> VVMSRGRIPRLGAAVLVALTTAAAACGADSQGLVVSFYTPATDGATFTAIAQRCNQQFGGRFTIAQVSLPRSPNEQRLQLARRLTGNDRTLDVMALDVVWTAEFAEAGWALPLSDDPAGLAENDAVADTLPGPLATAGWNHKLYAAPVTTNTQLLWYRPDLVNSPPTDWNAMIAEAARLHAAGEPSWIAVQANQGEGLVVWFNTLLVSAGGSVLSEDGRHVTLTDTPAHRAATVSALQILKS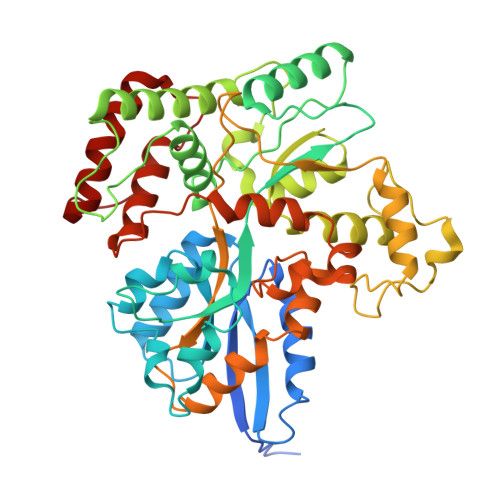VATTPGADPSITRTEEGSARLAFEQGKAALEVNWPFVFASMLENAVKGGVPFLPLNRIPQLAGSINDIGTFTPSDEQFRIAYDASQQVFGFAPYPAVAPGQPAKVTIGGLNLAVAKTTRHRAEAFEAVRCLRDQHNQRYVSLEGGLPAVRASLYSDPQFQAKYPMHAIIRQQLTDAAVRPATPVYQALSIRLAAVLSPITEIDPESTADELAAQAQKAIDGMGLLP> DVYQEPTDPKFPQQWYLSGVTQRDLNVKAAWAQGYTGHGIVVSILDDGIEKNHPDLAGNYDPGASFDVNDQDPDPQPRYTQMNDNRHGTRCAGEVAAVANNGVCGVGVAYNARIGGVRMLDGEVTDAVEARSLGLNPNHIHIYSASWGPEDDGKTVDGPARLAEE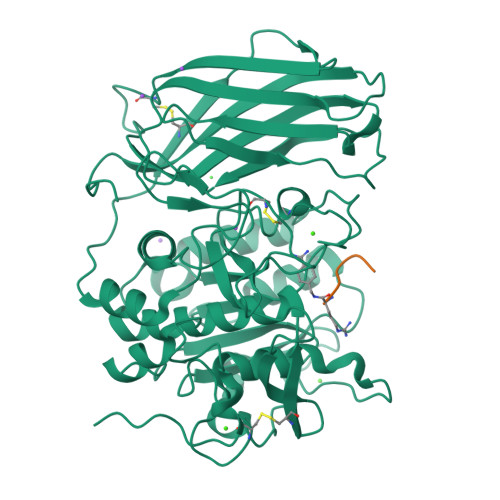AFFRGVSQGRGGLGSIFVWASGNGGREHDSCNCDGYTNSIYTLSISSATQFGNVPWYSEACSSTLATTYSSGNQNEKQIVTTDLRQKCTESHTGTSASAPLAAGIIALTLEANKNLTWRDMQHLVVQTSKPAHLNANDWATNGVGRKVSHSYGYGLLDAGAMVALAQNWTTVAPQRKCIIDILTEPKDIGKRLEVRKTVTACLGEPNHITRLEHAQARLTLSYNRRGDLAIHLVSPMGTRSTLLAARPHDYSADGFNDWAFMTTHSWDEDPSGEWVLEIENTSEANNYGTLTKFTLVLYGTASGSLVPRGSHHHHHH;> RRRVRX>GTSQVINGEMQFYARAKLFYQEVPATEEGMMGNFIELSSPDIQASQKFLRKFVGGPGRAGTDCALDCGSGIGRVSKHVLLPVFNSVELVDMMESFLLEAQNYLQVKGDKVESYHCYSLQEFTPPFRRYDVIWIQWVSGHLTDKDLLAFLSRCRDGLKENGIIILKDNVAREGCILDLSDSSVTRDMDILRSLIRKSGLVVLGQEKQDGFPEQCIPVWMFALH[2x];>[2x]XPKRIA

In order to unravel the molecular basis of the substrate and product specificity of NTMT2, we determine the X-ray crystal structures of NTMT2 in binary complex with SAM, as well as in ternary complex with SAH and an RCC1-derived peptide (SPKRIA). In addition, NTMT2 contains two auxiliary regions: an N-terminal α-lid (η1, α1–α2), and a β-lid (β6–β7) inserted between β5 and α8. These two lids cover the core domain that contributes to the substrate recognition. We also identify that N89 serves as a gatekeeper residue to control the entry of substrate into the active pocket.

To determine the molecular basis of different product specificities between NTMT2 and NTMT1, we solved crystal structures of the NTMT2-SAM binary complex and the NTMT2-SAH-SPKRIA peptide  ternary complex. Despite that an unmethylated peptide was used for crystallization, a methylated α-amino group in the N-terminus of the peptide was traced in the crystal structure. Our ternary complex structure shows that, like in NTMT1, the substrate peptide is deeply inserted into the binding pocket through hydrophilic and hydrophobic interactions, and the α-amine of the first residue (S1) points towards the sulfur atom of SAH. In the NTMT2 complex, S1 fits snugly into the channel, where the main-chain O atom is anchored by N223 in NTMT2 (N168 in NTMT1) through hydrogen bonding (Supplementary 2b). The substrate residue P2 is sandwiched by the aromatic side chains of W191 and F90. The ε-amine of substrate K3 interacts with two aspartates in both NTMT1 and NTMT2 structures. In NTMT2, the main-chain N and O atoms of K3 are involved in a water-mediated hydrogen bond with the side chain of N223 and a direct hydrogen bond with the main chain of I270, respectively. Substrate residues downstream of the S-P-K motif protrude from the pocket on the surface of NTMT2, indicating that they are not essential for the recognition. Indeed, the fourth residue R4 is not involved in direct interaction and the main chain of the fifth residue I5 is accommodated by Q268. The NTMT2-SAM binary complex subtly differs from the NTMT2-SAH-SPKRIA ternary complex in that the turn of the β-lid of the ternary complex is shifted closer to the catalytic core, which facilitates hydrogen bonding between substrate K3 and both D232 and D235 of NTMT2.>[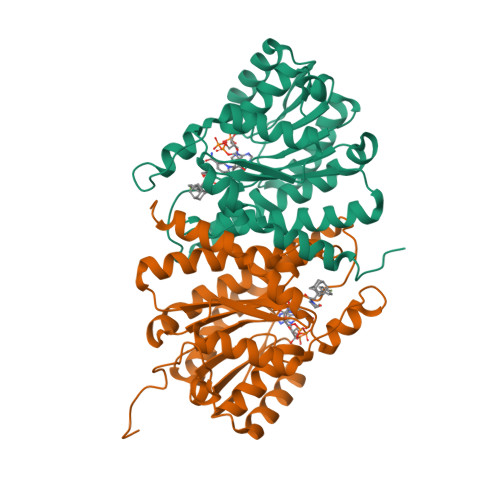4x]GSHMASMTGGQQMGRGSNEEFRPEMLQGKKVIVTGASKGIGREMAYHLAKMGAHVVVTARSKETLQKVVSHCLELGAASAHYIAGTMEDMTFAEQFVAQAGKLMGGLDMLILNHITNTSLNLFHDDIHHVRKSMEVNFLSYVVLTVAALPMLKQSNGSIVVVSSLAGKVAYPMVAAYSASKFALDGFFSSIRKEYSVSRVNVSITLCVLGLIDTETAMKAVSGIVHMQAAPKEECALEIIKGGALRQEEVYYDSSRWTTLLIRNPCRKILEELYSTSYNMDRFINK>MSGSHHHHHHSGSMSERPSDLVVNRLVLFVVKGTATSTHNTVKPLILLEELGVPHDIYVVEKVSAPWFSEINPHKMVPAILDRSPDGRDTLRAWEST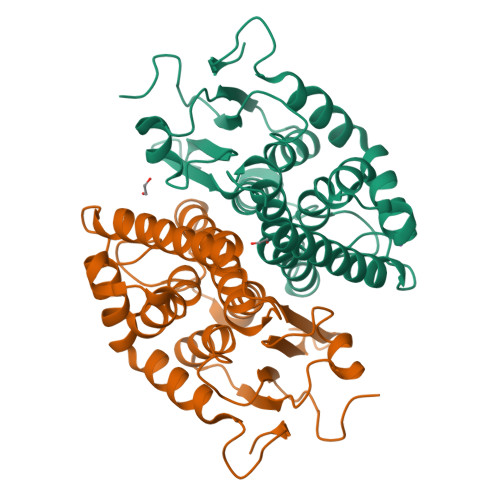STLMYIADAYDKDGTFGGRNVQERSEINNWLTLHTAALGPTAAYWLYFYKLHPEKLPKTIEKLRSNITVQYDILERRLNEPGQQYLALKDRPTIADIATLPFAMKSTAELFGLEFEKWPKLQEWSVRMGEREAVKRAWQRVAGFGHGEKEYGMLEA[6x]>[8x]SAAATQAVPAPNQQPEVFCNQIFINNEWHDAVSRKTFPTVNPSTGEVICQVAEGDKEDVDKAVKAARAAFQLGSPWRRMDASHRGRLLNRLADLIERDRTYLAALETLDNGKPYVISYLV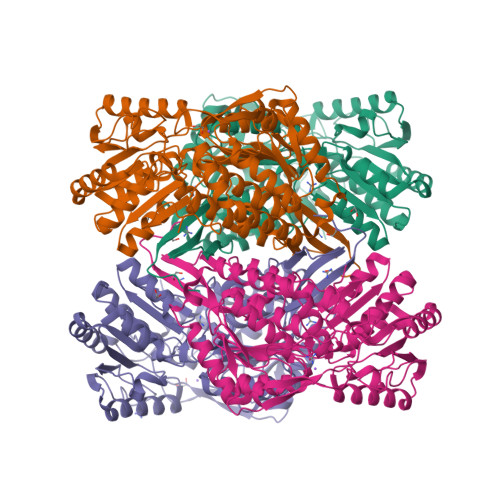DLDMVLKCLRYYAGWADKYHGKTIPIDGDFFSYTRHEPVGVCGQIIPWNFPLLMQAWKLGPALATGNVVVMKVAEQTPLTALYVANLIKEAGFPPGVVNIVPGFGPTAGAAIASHEDVDKVAFAGSTEIGRVIQVAAGSSNLKRVTLELGGKSPNIIMSDADMDWAVEQAHFALFFNQGQCCCAGSRTFVQEDIYDEFVERSVARAKSRVVGNPFDSKTEQGPQVDETQFKKILGYINTGKQEGAKLLCGGGIAADRGYFIQPTVFGDVQDGMTIAKEEIFGPVMQILKFKTIEEVVGRANNSTYGLAAAVFTKDLDKANYLSQALQAGTVWVNCYDVFGAQSPFGGYKMSGSGRELGEYGLQAYTEVKTVTVKVPQKNS> MSTKVKKTTQLK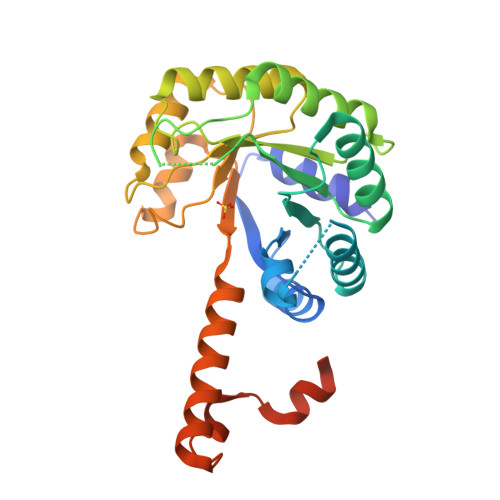QMLNSKDLEFIMEAHNGLSARIVQEAGFKGIWGSGLSVSAQLGVRDSNEASWTQVVEVLEFMSDASDVPILLDADTGYGNFNNARRLVRKLEDRGVAGACLEDKLFPKTNSLHDGRAQPLADIEEFALKIKACKDSQTDPDFCIVARVEAFIAGWGLDEALKRAEAYRNAGADAILMHSKKADPSDIEAFMKAWNNQGPVVIVPTKYYKTPTDHFRDMGVSMVIWANHNLRASVSAIQQTTKQIYDDQSLVNVEDKIVSVKEIFRLQRDDELVQAEDKYLPKN>[5x]PSESADPHELNEPRILTTDREAVAVAFSPGGSLLAGGSGDKLIHVWDVASGDELHTLEGHTDWVRAVAFSPDGALLASGSDDATVRLWDVAAAEERAVFEGHTHYVLDIAFSPDGSMVASGSRDGTARLWNVATGTEHAVLKGHTDYVYAVAFSPDGSMVASGSRDGTIRLWDVATGKERDVLQAPAENVVSLAFSPDGSMLVHGSDSTVHLW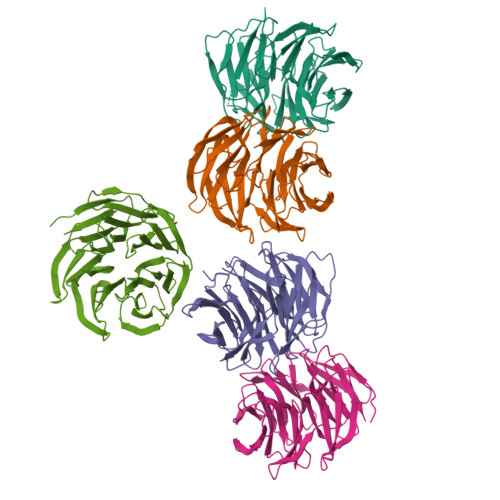DVASGEALHTFEGHTDWVRAVAFSPDGALLASGSDDRTIRLWDVAAQEEHTTLEGHTEPVHSVAFHPEGTTLASASEDGTIRIWPIATE> GHMKRFNVLKYIRTTKANIQTIAMPLTTKPLSLKINAALFDVDGTIIISQPAIAAFWRDFGKDKPYFDAEHVIHISHGW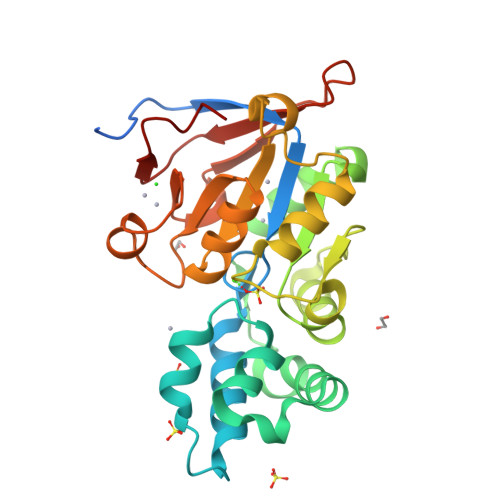RTYDAIAKFAPDFADEEYVNKLEGEIPEKYGEHSIEVPGAVKLCNALNALPKEKWAVATSGTRDMAKKWFDILKIKRPEYFITANDVKQGKPHPEPYLKGRNGLGFPINEQDPSKSKVVVFEDAPAGIAAGKAAGCKIVGIATTFDLDFLKEKGCDIIVKNHESIRVGEYNAETDEVELIFDDYLYAKDDLLKWGS>MKVGIVGSGMVGSATAYALALLGVAREVVLVDLDRKLAQAHAEDILHATPFAHPVWVRAGSYGDLEGARAVVLAAGVAQRPGETRLQLLDRNAQVFAQVVPRVLEAAP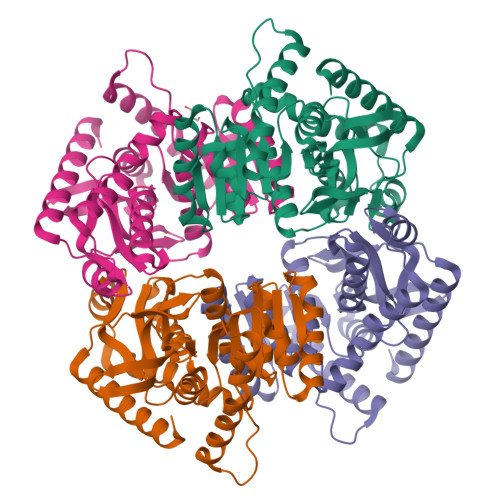EAVLLVATNPVDVMTQVAYRLSALPPGRVVGSGTILDTARFRALLAEHLRVAPQSVHAYVLGEHGDSEVLVWSSAQVGGVPLLEFAEARGRALSPEDRARIDEGVRRAAYRIIEGKGATYYGIGAGLARLVRAILTDEKGVYTVSAFTPEVEGVLEVSLSLPRILGAGGVEGTVYPSLSPEEREALRRSAEILKEAAFALGF[4x]GBS expresses three structurally distinct pilus types, each containing at least two antigens capable of eliciting protective immunity in mouse models, confirming a key role in bacterial pathogenesis. The three GBS pilus types are coded by distinct genomic loci containing features typical of Gram-positive pilus islands (PIs). These islands, named PI-1, PI-2a and PI-2b, encode three structural pilus proteins, corresponding to the major pilus subunit (backbone protein, BP) that forms the pilus shaft and two ancillary proteins that appear to be located at the pilus tip (AP1) and at the base (AP2) as anchor protein of the pilus to the bacterial cell-wall. Prior to the discovery of pilus-structures in Gram-positive bacteria, the backbone protein of pilus 2b (BP-2b) was described as a GBS surface invasin (named surface protein of GBS 1, Spb1), due to its ability to promote invasion of epithelial cells. Here we report the structural and functional characterization of the backbone protein of pilus 2b (BP-2b).

We solved the X-ray structure of a fragment of the protein (lacking the N-terminal first 184 residues) encompassing domains D2 and D3. Both domains revealed an IgG-like fold organization, typical of the pilin subunits, and the presence of internal isopeptide bonds. Pilus Island 2b (PI-2b) has been commonly found in the epidemiologically relevant GBS serotype III-ST-17 lineage. While the assembly of the well characterized GBS pili 1 and 2a occur following the classical model, the pilus 2b seems to differ slightly: the pilus 2b components do not contain the canonical conserved primary sequence of the pilin motif described for pilus polymerization in Gram-positive bacteria, making difficult the identification of the key residues involved in pilus assembly. Finally, by site-directed mutagenesis and complementation studies in GBS strains we identified the non-canonical residues/motives essential for the BP-2b protein polymerization. Using the three-dimensional information we generated the single structurally well-defined domains as recombinant proteins and compared their protective immunity with the full length protein in a well-established mouse model.

> MGGKTVDQKTYSVGDTVKYTITYKNAVNYHGTEKVYQYVIKDTMPSASVVDLNEGSYEVTITDGSGNITTLTQGSEKATGKYNLLEENNNFTITIPWAATNTPTGNTQNGANDDFFYKGINTITVTYTGVLKSGAKPGSADLPENTNIATINPNTSNDDPGQKVTVRDGQITIKKIDGSTKASLQGAIFVLKNATGQFLNFNDTNNVEWGTEANATEYTTGADGIITITGLKEGTYYLVEKKAPLGYNLLDNSQKVILGDGATDTTNSDNLLVNPTVENNKGTELPSHHHHH>MNHKVHHHHHHIEGRHMTELKSKFVKVYSVLKKELLHDSAFGLTDDSRNWVERIMDYNVPGGKLNRGLSVVDSYKLLRELTGGKSELSDDEIFLASVLGWSVEWIQAYFLVLDDIMDHSHTRRGHPCWFRLPKVGMIAINDGLILRNHVPRILRTHFQTEHYYLQLVDLFHEVECQTIAGQMLDLITTLAGEINLSSYSLPVYQQITLSKTSYYSFYLPVACALVMLGENLESHDDMKDILLEMGTYFQVQDDYLDCFGDPEVIGKIGTDIEDNKC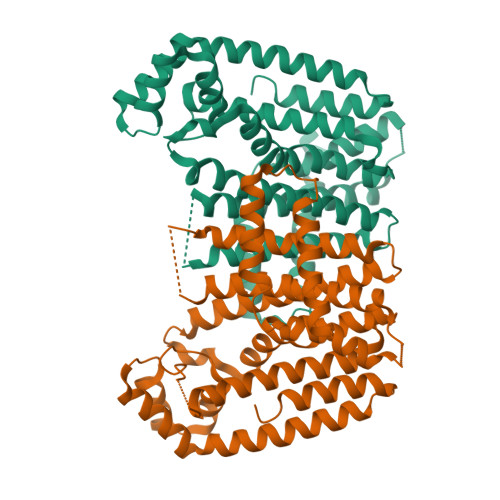TWLVVQALEHCNEEQKKLLYDNYGRKDPKQVAKVKELYKTLNLEDLFTQYENKTCKKLTKSIEALPNVAVQAVLKSFLAKIHKRLK[2x]>SMQSSKRSSRSVEDDKEGHLVCRIGDWLQERYEIVGNLGEGTFGKVVECLDHARGKSQVALKIIRNVGKYREAARLEINVLKKIKEKDKENKFLCVLMSDWFNFHGHMCIAFELLGKNTFEFLKENNFQPYPLPHVRHMAYQ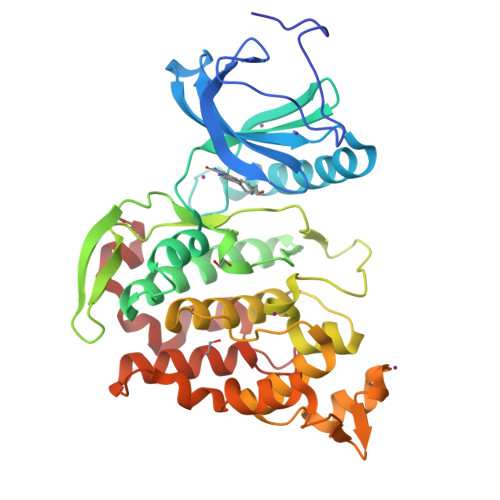LCHALRFLHENQLTHTDLKPENILFVNSEFETLYNEHKSCEEKSVKNTSIRVADFGSATFDHEHHTTIVATRHYRPPEVILELGWAQPCDVWSIGCILFEYYRGFTLFQTHENREHLVMMEKILGPIPSHMIHRTRKQKYFYKGGLVWDENSSDGRYVKENCKPLKSYMLQDSLEHVQLFDLMRRMLEFDPAQRITLAEALLHPFFAGLTPEERSFHT[2x]>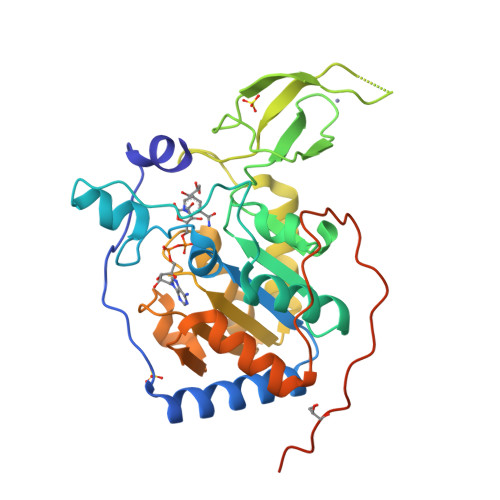[6x]VNYAAGLSPYADKGKCGLPEIFDPPEELERKVWELARLVWQSSSVVFHTGAGISTASGIPDFRGPHGVWTMEERGLAPKFDTTFESARPTQTHMALVQLERVGLLRFLVSQNVDGLHVRSGFPRDKLAELHGNMFVEECAKCKTQYVRDTVVGTMGLKATGRLCTVAKARGLRACRGELRDTILDWEDSLPDRDLALADEASRNADLSITLGTSLQIRPSGNLPLATKRRGGRLVIVNLQPTKHDRHADLRIHGYVDEVMTRLMKHLGLEIPAWDGPRVLERALPPLPRPPTPKLEPKEESPTRINGSIPAGPKQE>[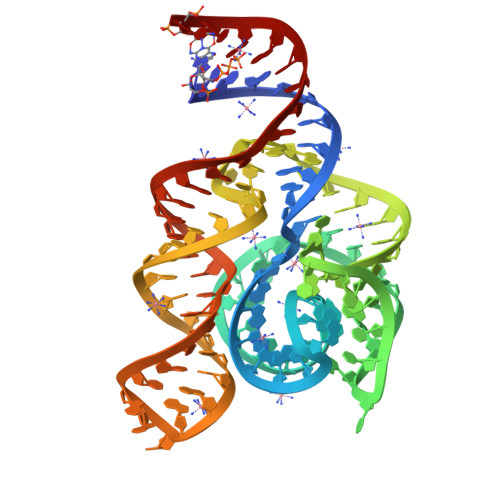2x]GGCCGUGCUAAGCGGGGAGGUAGCGGUGCCCUGUACCUGCAAUCCGCUCUAGCAGGGCCGAAUCCCUUCUCGAGGUGGUAACAUCGACAGAAGGUGCACGGUC>GMNQAMDTKQIAPFTLALPEGEALPLVCDSPHSGTFYPADFGAVVAPERLRGGEDTHVDALWEAVPRVGGTLLAATFPRVYIDPNRMLDDIDPAQLEGPWPTPLAPGEKTRLGYGLIWSNVDAATPIYDRKLTVAEVQRRINRYYRPYHAALTEAVEGAYQRFGAVWHLNLHSMPNNAYERLKIQSPRPLADFVLGDRDGTTCEPGLVDLVERELREKGYTVARNDPYKGVQLIAQIGRPAERRNSLQIEIRRPLYMEEGTRERNEGFATLQ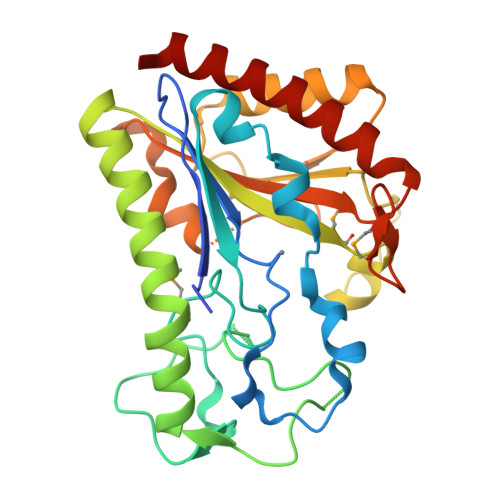RDLTLLTLRIAEYVRRGV[2x]Originally discovered in the circulation of pregnant women as a protein secreted by placental trophoblasts, the metalloprotease pregnancy-associated plasma protein A (PAPP-A) is also widely expressed by many other tissues. It cleaves insulin-like growth factor-binding proteins (IGFBPs) to increase the bioavailability of IGFs and plays essential roles in multiple growth-promoting processes. While the vast majority of the circulatory PAPP-A in pregnancy is proteolytically inactive due to covalent inhibition by proform of eosinophil major basic protein (proMBP), the activity of PAPP-A can also be covalently inhibited by another less characterized modulator, stanniocalcin-2 (STC2). Here we present two cryo-EM structures of endogenous purified PAPP-A in complex with either proMBP or STC2. Both modulators form 2:2 heterotetramer with PAPP-A and establish extensive interactions with multiple domains of PAPP-A that are distal to the catalytic cleft.

To assess the molecular mechanism(s) subserving PAPP-A activity and the modulation of proMBP, we purified endogenous PAPP-A·proMBP complex from pregnant human plasma and determined its cryo-EM structure. The presence of full-length proMBP was confirmed by western blotting using a proMBP-specific antibody and non-reduced gels showed a major heterotetrameric form for PAPP-A·proMBP. The cryo-EM analysis generated an initial dimeric 3D map at 3.64 Å resolution, and C2-symmetry expansion was subsequently applied to obtain a final 3.45-Å monomeric half map, which enabled de novo modeling of most of the PAPP-A residues. The dimer cryo-EM map contains two copies of the full-length mature PAPP-A and two copies of proMBP, exhibiting an overall butterfly-shaped structure with a dimension of 230 Å × 110 Å × 90 Å. As shown in our structure, proMBP itself is a monomer. In the PAPP-A·proMBP complex, the binding of proMBP induces a nearly 30° rotation of the βBD towards the PD, generating an interface between the βBD and the C-terminal subdomain of PD. As a result, the relative orientation of the LGD, PD, and SD remains unchanged in the two complexes, forming a rigid core of PAPP-A; but the βBD, CCP, and CTD have drastic translational and rotational differences and thus constitute a movable region. The comparison of the two structures identified a twist motion for PAPP-A conformation similar to a “butterfly wing-flap”. Although the highly intrinsic flexibility at the interface between the two PAPP-A subunits results in a less resolvable density here, we still found that the dimeric interfaces contain not only the previously characterized intermolecular disulfide bond but also a strong hydrophobic pocket between the two βBD. While proMBP formed a 2:2 tetramer with WT PAPP-A (lane 4), it could only partially form a 1:1 dimer with C1130S variant (lane 5).

>MKLPLLLALLFGAVSALHLRSETSTFETPLGAKTLPEDEETPEQEMEETPCRELEEEEEWGSGSEDASKKDGAVESISVPDMVDKNLTCPEEEDTVKVVGIPGCQTCRYLLVRSLQTFSQAWFTCRRCYRGNLVSIHNFNINYRIQCSVSALNQGQVWIGGRITGSGRCRRFQWVDGSRWNFAYWAAHQPWSRGGHCVALCTRGGHWRRAHCLRRLPFICSY[2x];>[2x]MRLWSWVLHLGLLSAALGCGLAERPRRARRDPRAGRPPRPAAGPATCATRAARGRRASPPPPPPPGGAWEAVRVPRRRQQREARGATEEPSPPSRALYFSGRGEQLRLRADLELPRDAFTLQVWLRAEGGQRSPAVITGLYDKCSYISRDRGWVVGIHTISDQDNKDPRYFFSLKTDRARQVTTINAHRSYLPGQWVYLAATYDGQFMKLYVNGAQVATSGEQVGGIFSPLTQKCKVLMLGGSALNHNYRGYIEHFSLWKVARTQREILSDMETHGAHTALPQLLLQENWDNVKHAWSPMKDGSSPKVEFSNAHGFLLDTSLEPPLCGQTLCDNTEVIASYNQLSSFRQPKVVRYRVVNLYEDDHKNPTVTREQVDFQHHQLAEAFKQYNISWELDVLEVSNSSLRRRLILANCDISKIGDENCDPECNHTLTGHDGGDCRHLRHPAFVKKQHNGVCDMDCNYERFNFDGGECCDPEITNVTQTCFDPDSPHRAYLDVNELKNILKLDGSTHLNIFFAKSSEEELAGVATWPWDKEALMHLGGIVLNPSFYGMPGHTHTMIHEIGHSLGLYHVFRGISEIQSCSDPCMETEPSFETGDLCNDTNPAPKHKSCGDPGPGNDTCGFHSFFNTPYNNFMSYADDDCTDSFTPNQVARMHCYLDLVYQGWQPSRKPAPVALAPQVLGHTTDSVTLEWFPPIDGHFFERELGSACHLCLEGRILVQYASNASSPMPCSPSGHWSPREAEGHPDVEQPCKSSVRTWSPNSAVNPHTVPPACPEPQGCYLELEFLYPLVPESLTIWVTFVSTDWDSSGAVNDIKLLAVSGKNISLGPQNVFCDVPLTIRLWDVGEEVYGIQIYTLDEHLEIDAAMLTSTADTPLCLQCKPLKYKVVRDPPLQMDVASILHLNRKFVDMDLNLGSVYQYWVITISGTEESEPSPAVTYIHGSGYCGDGIIQKDQGEQCDDMNKINGDGCSLFCRQEVSFNCIDEPSRCYFHDGDGVCEEFEQKTSIKDCGVYTPQGFLDQWASNASVSHQDQQCPGWVIIGQPAASQVCRTKVIDLSEGISQHAWYPCTISYPYSQLAQTTFWLRAYFSQPMVAAAVIVHLVTDGTYYGDQKQETISVQLLDTKDQSHDLGLHVLSCRNNPLIIPVVHDLSQPFYHSQAVRVSFSSPLVAISGVALRSFDNFDPVTLSSCQRGETYSPAEQSCVHFACEKTDCPELAVENASLNCSSSDRYHGAQCTVSCRTGYVLQIRRDDELIKSQTGPSVTVTCTEGKWNKQVACEPVDCSIPDHHQVYAASFSCPEGTTFGSQCSFQCRHPAQLKGNNSLLTCMEDGLWSFPEALCELMCLAPPPVPNADLQTARCRENKHKVGSFCKYKCKPGYHVPGSSRKSKKRAFKTQCTQDGSWQEGACVPVTCDPPPPKFHGLYQCTNGFQFNSECRIKCEDSDASQGLGSNVIHCRKDGTWNGSFHVCQEMQGQCSVPNELNSNLKLQCPDGYAIGSECATSCLDHNSESIILPMNVTVRDIPHWLNPTRVERVVCTAGLKWYPHPALIHCVKGCEPFMGDNYCDAINNRAFCNYDGGDCCTSTVKTKKVTPFPMSCDLQGDCACRDPQAQEHSRKDLRGYSHG>[2x]DADKLPHTKVTLVAPPQVHPHEQATKSGPKVVEFTMTIEEKKMVIDDKGTTLQAMTFNGSMPGPTLVVHEGDYVQLTLVNPATNAMPHNVDFHGATGALGGAKLTNVNPGEQATLRFKADRSGTFVYHCAPEGMVPWHVVSGMSGTLMVLPRDGLKDPQGKPLHYDRAYTIGEFDLYIPKGPDGKYKDYATLAESYGDTVQVMRTLTPSHIVFNGKVGALTGANALTAKVGETVLLIHSQANRDTRPHLIGGHGDWVWETGKFANPPQRDLETWFIRGGSAGAALYTFKQPGVYAYLNHNLIEACELGAAGHIKVEGKWNDDLMKQIKAPAPIPR

Copper-containing nitrite reductases (CuNiRs) catalyse the one-electron reduction of nitrite to nitric oxide: NO2−+2H++e− ↔ NO+H2O, a step in the microbial ATP-generating respiratory dentrification pathway. CuNiRs are trimeric and each monomer has two characteristic β-sandwich cupredoxin domains that contain a T1Cu centre with (Cys–Met–His2) ligation. The active site is a T2Cu with (His3–H2O) ligation, which is situated at the interface between two adjacent monomers in a cleft ~12 Å from the protein surface. Electrons produced during denitrification are donated to the T1Cu site by a partner redox protein and subsequently transferred via a 12.6-Å His–Cys bridge to the T2Cu centre in a proton-gated reaction.

Here we show that substitution of a surface residue (F306C) at the entrance of the channel of CuNiR results in an altered second sphere coordination of the active site Cu. Comparison of the crystallographic structures of the ‘as isolated’ (1.7 Å resolution) and substrate bound (1.75 Å resolution), allowed us to assess the effect of this substitution on the substrate access channel and its associated water network. The substitution did not change the highly ordered hydrogen bonded water network (Asp92–water–water–Ala131–Asn90–Asn107) from the T2Cu site to the protein surface that provides the major route of proton delivery to the active site. A notable feature of the channel was the presence of an additional water molecule hydrogen bonded to the liganded water of the T2Cu ion. This second water molecule has no counterpart in the numerous structures of other two domain CuNiRs, and presents an altered energy landscape for nitrite displacement of the Cu-coordinated water molecule during catalysis. Since the structure shows access to the substrate channel is enhanced, the weaker apparent affinity for nitrite may arise from the presence of the additional water in the second coordination sphere of the T2Cu stabilizing the coordinated water that nitrite needs to displace in order to bind. An additional contributing feature revealed by the structure is the positioning of the gatekeeper Asp92 residue in the ‘closed’ conformation that may result in a slower escape of NO from the active site pocket, resulting in a weaker apparent KM value for nitrite due to competitive binding of NO to T2Cu in the micro-reversibility of NiR function. The sensor loop10 (His94-Asp92-His89) that reports the status of the T2Cu site to the electron-donating T1Cu site remains unaltered. The space generated by the F306C mutation also allows an adjacent surface residue at the mouth of the channel, Met135, to adopt a dual conformation. Because access of both water and nitrite is enhanced, we attribute the 50-fold increase in apparent KM for nitrite not to there being more water to compete with, but rather arising from stabilization of the ligated water owing to its hydrogen bonding to W2, making it more difficult for nitrite to displace.> GAMGRPALEAVTRPERVPLTARQLRAWLLARPSEETRGRHLSVALRLRGRLDVAALEAALRDVAARHEILRTTFPGDAQTVHQHIHDAAPVRLTPVPATEEDLPARLAERGEQLFDLTRDMPWRCELFALSEKEHVLSVTVHRIAADDDSMDVFFRDLAAAYGARRAGRAPERAPLALQFADYAIWEQRLLDGEREQDSLINDQITFWRNHLAGIDQETVLPFDRARPAIPSRRAGTVALRLDAGP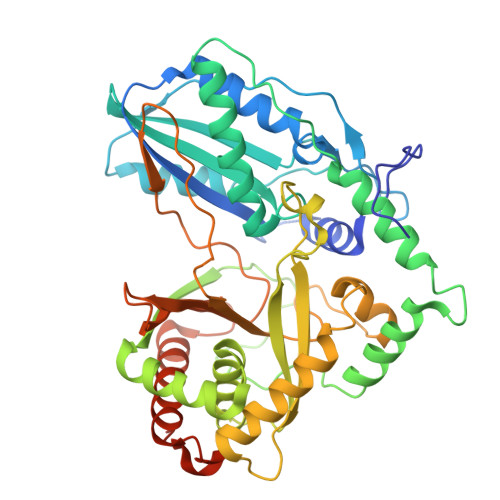HARLAEAVESAGADMPQLVQAALAMLLTRYGAGTDLVIGTTLPRDEDLIDLEPMIGPFARPFPVRTDLSADPTFLEVVARVQEAVREARQHLDVPFEKIPELLALPGSLSRHPVYQVGLQVREEDNGAWDAAELPALRTSVEPTGVEAIELDLAFALTERRNDDDDEDGIEGALHYAADLFDHDTAASLARRLVRVLEQVAEDPGRRISDLDILLDDAERGAPLESAWSHPQFEK> ETRPNHTIYINNLNEKIKKDELKKSLHAIFSRFGQILDILVSRSLKMRGQAFVIFKEVSSATNALRSMQGFPFYDKPMRIQY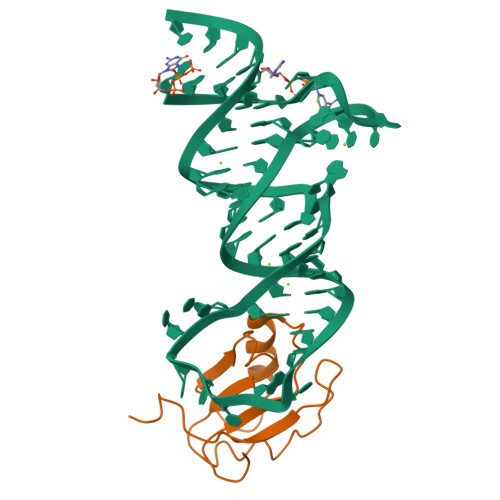AKTDSDIIAK> GQAREALELAIRGGFHAYLVGPPSLGKHEALLAYLSTQSVETPPDLLYVPLSERKVAVMTLPSGQEIHLAEAVEGLLLEVNRLDELFRQGSFLREKTQLEARFKEAREQQLEALRREAQEAGFALSTNGERLELTGPGPVPAELSARLEEVTLGSMAASAELEVALRRLRRDWALHYLNNRFEPLFQRFPQARAYLEALRARLARYAETGEPLDPAQWRPNLLTSSSSGTPPPIVYEPYATAPRLFGRLDYLVDRGVWSTNVSLIRPGAVHRAQGGYLILDALSLKREGTWEAFKRALRNGQVEPVTEPQAPAGLEVEPFPIQMQVMLVGTPEAFEGLE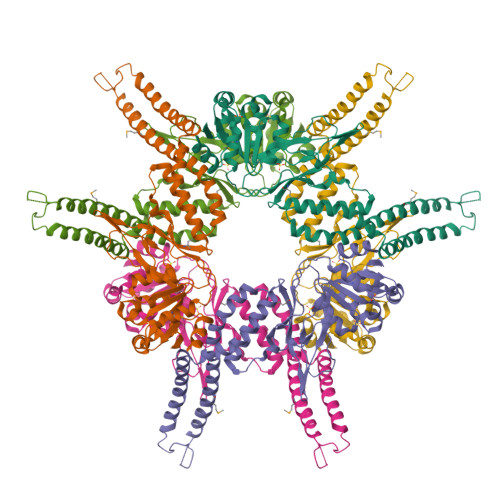EDPAFSELFRIRAEFS Base-J (β-D-glucopyranosyloxymethyluracil) is a modified DNA nucleotide that replaces 1% of thymine in kinetoplastid flagellates. The biosynthesis and maintenance of base-J depends on the base-J-binding protein 1 (JBP1) that has a thymidine hydroxylase domain and a J-DNA-binding domain (JDBD). JBP1 specifically recognizes base-J-containing double-stranded DNA (J-DNA) through a JDBD which has been structurally characterized. In the context of JBP1, JDBD recognizes base-J and then probably invokes a conformational change in JBP1 (25, 26), enabling the THD to initiate the biosynthesis of base-J on a thymine 13 base pairs downstream the complementary DNA strand (J + 13′ position).

Notably, the crystal structure of the JDBD had a missing loop of eight residues (529–537) between helices α4 and α5, including the Arg532 that is important for DNA binding. Remarkably, in one of numerous datasets that have been obtained during the course, the missing density for the loop 529–537 was observed. As this loop follows the α4 recognition helix and harbors the Arg532 residue which affects DNA binding, the diffraction data from the CSHL 2018 course were reprocessed, and the model was rebuilt and refined. The B factors in the loop range between 53.5 and 125.2 (mean 91.6) compared with a mean of 65.3 for the JDBD structure excluding the five α-helices. There are no crystal contacts observed for this loop, and there are no substantial differences in crystal properties overall. Thus, it remains unclear why the 529–537 loop is ordered in the new structure and not in previous experiments. The final structure was validated using MolProbity and it belongs to the 100th percentile, with a Ramachandran Z-score of −0.98 ± 0.72. Here, we present a crystal structure of the JDBD including a previously disordered DNA-contacting loop and use it as starting point for molecular dynamics simulations and computational docking studies to propose recognition models for JDBD binding to J-DNA. In this predicted model, JDBD shows a similar overall fold when compared with our new crystal structure, with a noticeable difference in the loop between the α4 and α5 helices, that we found ordered in the new JDBD crystal structure.

> TNLMVSTAVEKKKYLDSEFLLHCISAQLLDMWKQARARWLELVGKEWAHMLALNPERKDFLWKNQSEMNSAFFDLCEVGKQVMLGLLGKEVALPKEEQAFWIMYAVHLSAACAEELHMPEVAMSLRKLNVKLKDFNFGGTRYFKDMPPEEKKRRMERKQRIEEARRHGMP>[10x]QANLMRLKSDLFNRSPMYPGPTKDDPLTVTLGFTLQDIVKVDSSTNEVDLVYCEQQRWKLNSLMWDPNEYGNITDFRTSAADIWTPDITAYSSTRPVQVLSPQIAVVT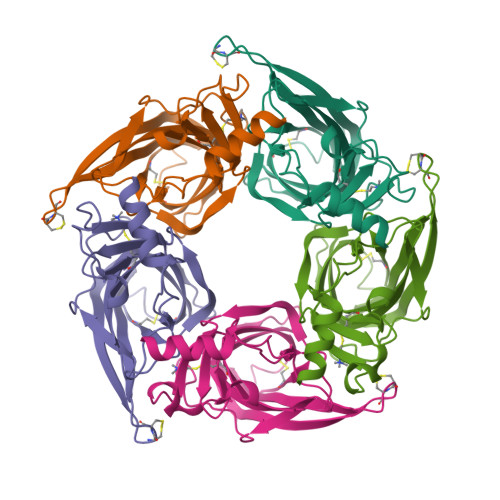HDGSVMFIPAQRLSFMCDPTGVDSEEGVTCAVKFGSWVYSGFEIDLKTDTDQVDLSSYYASSKYEILSATQTRQVQHYSCCPEPYIDVNLVVKFRERRAGNGFFRNLFD>MSNLPHEPEFEQAYKELASTLENSTLFQKNPEYRKALAVVSVPERVIQFRVVWEDDAGNVQVNRGFRVQFNSALGPYKGGLRFHPSVNLSILKFLGFEQIFKNALTGLNMGGGKGGSDFDPKGKSDNEIRRFCVSFMTELCKHIGADTDVPAGDIGVTGREVGFLFGQYRKIRNQWEGVLTGKGGSWGGSLIRPEATGYGVVYYVEHMIAHATNGQESFKGKRVAISGSGNVAQYAALKVIELGGSVVSLSDSQGSLIINGEGSFTPEEIELIAQTKVERKQLASIVGAAPFSDANKFKYIAGARPWVHVGKVDVALPSATQNEISGEEAQVLINAGCKFIAEGSNMGCTQEAIDTFEAHRTANAGAAAIWYAPGKAANAGGVAVSGLEMAQNSARLSWTSEEVDARLKDIMRDCFKNGLETAQEYATPAEGVLPSLVTGSNIAGFTKVAAAMKDQGD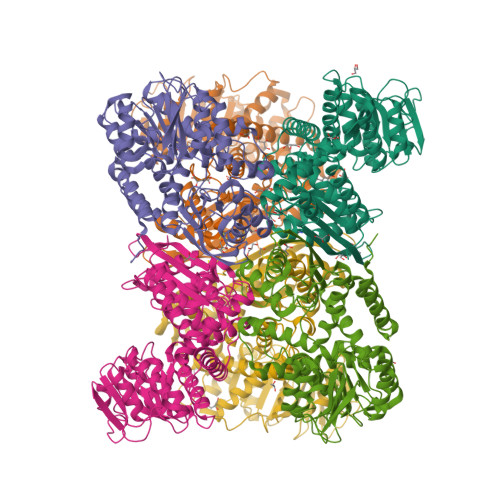WW[6x]>MLTEAQMASTANLMRKMCQPKTKVTDEQINNFHKGVFDDDKKMMCYMNCILETMKIIKNGKLDMSAVEQQMPTL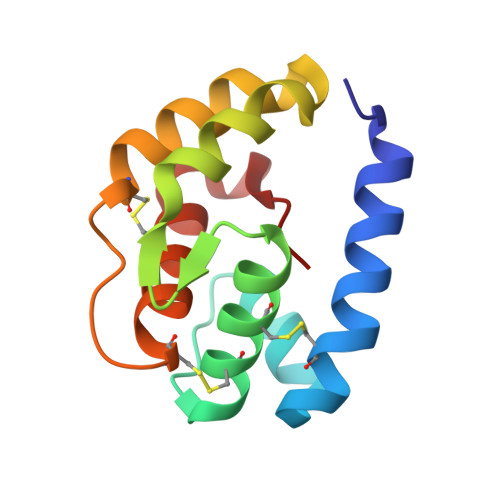PKKYQESTKKSIEECKSADTGDKCEPAYNFAKCLYLSNPEMYFLP[2x]> GISQPQEPELMNANPAPPPAPSQQINLGPSSNPHAKPSDFHFLKVIGKGSFGKVLLARHKAEEVFYAVKVLQKKAILKKKEEKHIMSERNVLLKNVKHPFLVGLHFSFQTADKLYFVLDYINGGELFYHLQRERCFLEPRARFYAAEIASALGYLHSLNIVYRDLKPENILLDSQGHIVLTDFGLCKENIEHNSTTSTFCGTPEYLAPEVL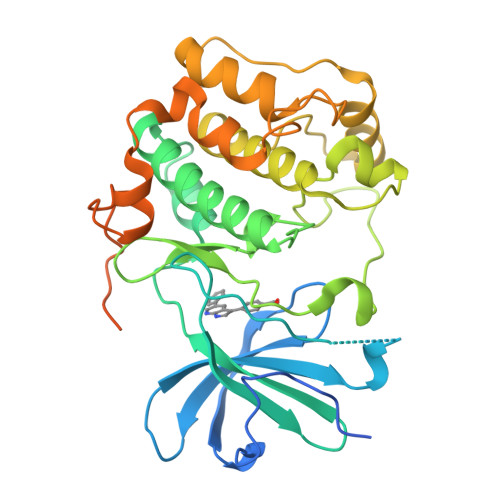HKQPYDRTVDWWCLGAVLYEMLYGLPPFYSRNTAEMYDNILNKPLQLKPNITNSARHLLEGLLQKDRTKRLGAKDDFMEIKSHVFFSLINWDDLINKKITPPFNPNVSGPNDLRHFDPEFTEEPVPNAIGKAPDSVLVTASVKEAAEAFLGFSYAPPTDSFL> MNIFRLTGDLSHLAAIIILLLKIWKSRSCAGISGKSQLLFALVFTTRYLDLFTSFISLYNTSMKLIYIACSYATVYLIYMKFKATYDGNHDTFRVEFLIVPVGGLSFLVNHDFSPLEILWTFSIYLESVAILPQLFMISKTGEAETITTHYLFFLGLYRALYLVNWIWRYYFEGFFDLIAVVAGVVQTVLYCDFFYLYVTKVLKGKKLSLPA;> TAEHDEF

The selective capture and retrieval of ER luminal proteins is controlled by the KDEL receptor (KDELR), which recognizes a specific ER-retrieval signal sequence (ERS) Lys-Asp-Glu-Leu (KDEL) at the C terminus of cargo proteins. Crystal structures of the chicken KDELR revealed a seven transmembrane (TM) spanning integral membrane protein with structural homology to the PQ-loop superfamily of membrane transporters. In the mildly acidic environment of the Golgi, KDEL-containing ER luminal proteins bind the receptor with high affinity, which elicits a signal for the integration of receptor-cargo complexes into COPI vesicles. In contrast, the neutral pH of the ER results in cargo release and the subsequent relocation of the empty receptor back to the Golgi, resetting the retrieval cycle.

Given that the stability of the hydrogen bonding network largely determines the solvation free energy, we attempted to investigate if the phenylalanine variant at the −1 position would disrupt the water network. Though the hydrogen bond between the waters and the His12 or the C terminus is equally strong for HDEL and HDEF ERS sequences, the hydrogen bond between the two waters is much less stable in HDEF compared with HDEL. The W1 and W2 water molecules are observed in the binding site, consistent with our previous HDEL structure and computational analysis. In both structures, the space available for the two waters is very tight. Thus, a slight perturbation of the protein might compress the space and disrupt the inter-water hydrogen bond network. A leucine at the −1 position of the ERS, however, would have more flexibility to maintain the water network compared to a terminal phenylalanine, which, being more rigid, would not provide sufficient flexibility and thus result in a less stable water network. Supporting this hypothesis, the temperature factors, or B factors, of the terminal leucine in the HDEL structure are 51.3 vs. 38.2 Å2 for the HDEF structure, demonstrating that phenylalanine is held more rigidly. Additionally, the affinity for TAEHDEF is lower than for TAEHDEL (23 μM vs. 18 μM), consistent with these observations. In summary, it seems likely that the increased affinity observed for the TAEHDEL peptide over the TAEHDEF peptide is due to the increased flexibility of the leucine side chain that enables more optimal coordination of the water molecules with the carboxy-terminus of the peptide within the receptor and explains the reduced ability of the HDEF ERS to retain proteins in the cell-based retrieval assay. The −1 phenylalanine KDEF and HDEF variants were retained more efficiently than the alanine variants but less efficiently than when leucine is present, consistent with our PMF calculations.>[4x]MHHHHHHHHENLYFQGSKEKF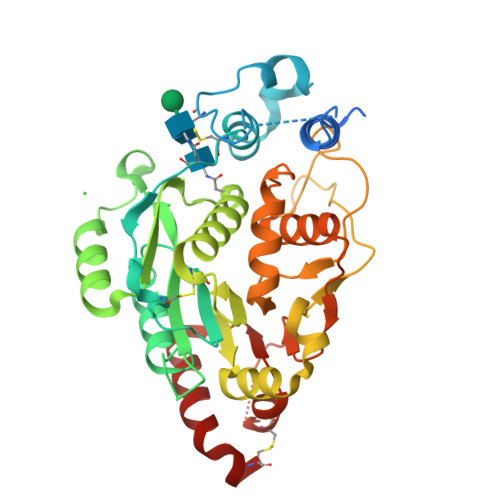WKISTPPEAYWNREQEKLNRQYNPILSMLTNQTGEAGRLSNISHLNYCEPDLRVTSVVTGFNNLPDRFKDFLLYLRCRNYSLLIDQPDKCAKKPFLLLAIKSLTPHFARRQAIRESWGQESNAGNQTVVRVFLLGQTPPEDNHPDLSDMLKFESEKHQDILMWNYRDTFFNLSLKEVLFLRWVSTSCPDTEFVFKGDDDVFVNTHHILNYLNSLSKTKAKDLFIGDVIHNAGPHRDKKLKYYIPEVVYSGLYPPYAGGGGFLYSGHLALRLYHITDQVHLYPIDDVYTGMCLQKLGLVPEKHKGFRTFDIEEKNKNNICSYVDLMLVHSRKPQEMIDIWSQLQSAHLKC>KPIEIIGAPFSKGQPRGGVEKGPAALRKAGLVEKLKETEYNVRDHGDLAFVDVPNDSPFQIVKNPRSVGKANEQLAAVVAETQKNGTISVVLGGDNSMAIGSISGHARVHPDLCVIWVDAHTDINTPLTTSSGNLHGQPVAFLLKE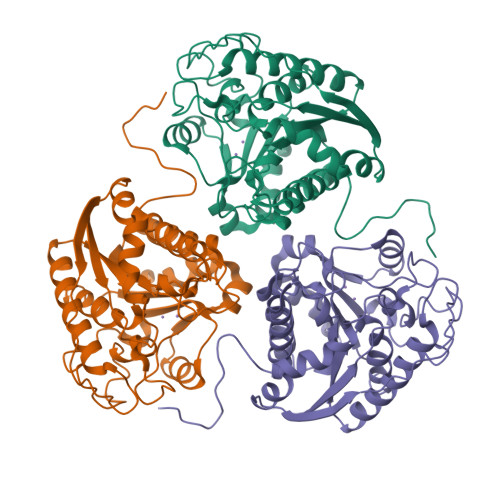LKGKFPDVPGFSWVTPCISAKDIVYIGLRDVDPGEHYIIKTLGIKYFSMTEVDKLGIGKVMEETFSYLLGRKKRPIHLSFDVDGLDPVFTPATGTPVVGGLSYREGLYITEEIYKTGLLSGLDIMEVNPTLGKTPEEVTRTVNTAVALTLSCFGTKREGNHKPETDYL[3x]> ASENIEVHMLNKGAEGAMVFEPAYIKANPGDTVTFIPVDKGHNVESIKDMI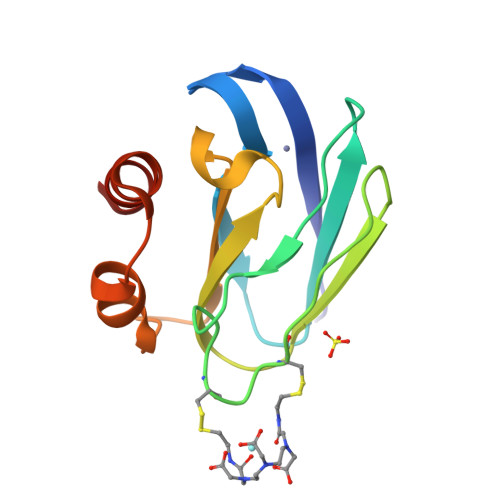PCGACKFKSKINENYVLTVTQPGAYLVKCTPHYAMGMIALIAVGDSPANLDQIVSAKKPKIVQERLEKVIASAK> MGSSHHHHHHSQDPNSLSNNISFFIDNSQTTAIEEIESELSSEKVDYIQEIGLVSFKNLDDSDRKFIGKYFNVSEGKKLPDFKPEEVNSSIL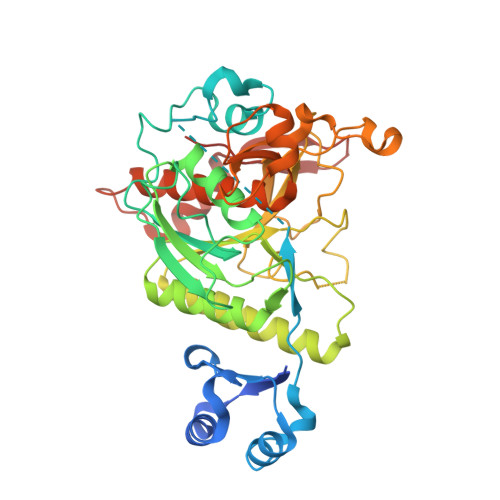NINILNKDFKSFNWPYKKILSHIDPVKEQLGKDITIALIDSGIDRLHPNLQDNNLRLKNYVNDIELDEYGHGTQVAGVIDTIAPRVNLNSYKVMDGTDGNSINMLKAIVDATNDQVDIINVSLGSYKNMEIDDERFTVEAFRKVVNYARKNNILIVASAGNESRDISTGNEKHIPGGLESVITVGATKKSGDIADYSNYGSNVSIYGPAGGYGDNYKITGQIDAREMMMTYYPTSLVSPLGKAADFPDGYTLSFGTSLATPEVSAALAAIMSKNVDNSKDSNEVLNTLFENADSFIDKNSMLKYKEVRIK> IVGGYTCGANTVPYQVSLNSGYHFCGGSLINSQWVVSAAHCYKSGIQVRLGEDNINVVEGNEQFISASKS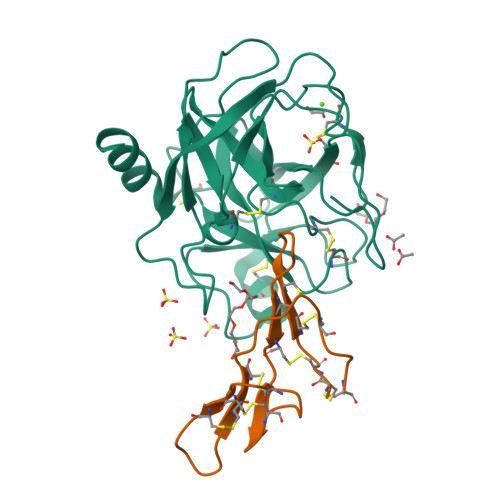IVHPSYNSNTLNNDIMLIKLKSAASLNSRVASISLPTSCASAGTQCLISGWGNTKSSGTSYPDVLKCLKAPILSDSSCKSAYPGQITSNMFCAGYLEGGKDSCQGDSGGPVVCSGKLQGIVSWGSGCAQKNKPGVYTKVCNYVSWIKQTIASN;> SGHHEDSTDEASESSKPCCDRCECTKSIPPQCRCSDVRLNSCHSACKSCACTFSIPAQCFCGDINDFCYKPCKSSHSDDDDWN>MKKGHHHHHHGSERTGTQPLGVQGLTEEQRMMIRELMDAQMKTFDTTFSHFKNFRLPGVLSSGCELPESLQAPSREEAAKWSQVRKDLCSLKVSLQLRGEDGSVWNYKPPADSGGKEIFSLLPHMADMSTYMFKGIISFAKVISYFRDLPIEDQISLLKGAAFELCQLRFNTVFNAETGTWECGRLSYCLEDTAGGFQQLLLEPMLKFHYMLKKLQLHEEEYVLMQAISLFSPDRPGVLQHRVVDQLQEQFAITLKSYIECNRPQPAHRF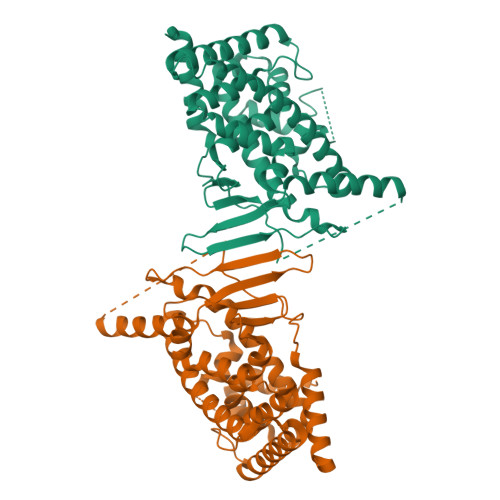LFLKIMAMLTELRSINAQHTQRALRIQDIHPFATPLMQELFGITGSSGGSGGSSHSSLTERHKILHRLLQEGSPSDITTLSVEPD[2x]>[6x]VFAEVPQAQPVLVFKLTADFREDPDPRKVNLGVGAYRTDDCHPWVLPVVKKVEQKIANDNSLNHEYLPILGLAEFRSCASRLALGDDSPALKEKRVGGVQSLGGAGALRIGADFLARWYNGTNNKNTPVYVSSPTWENHNAVFSAAGFKDIRSYRYWDAEKRGLDLQGFLNDLENAPEFSIVVLHACAHNPTGIDPTPEQWKQIASVMKHRFLFPFFDSAYQGFASGNLERDAW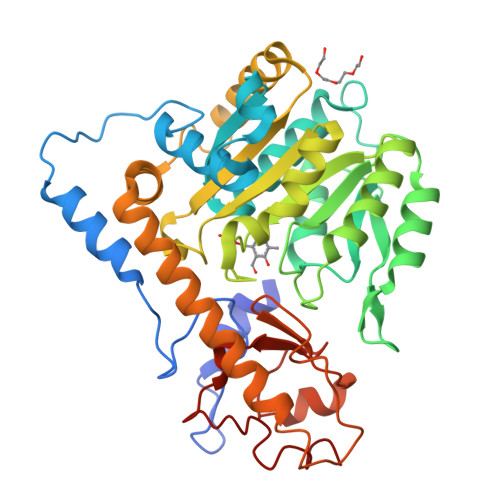AIRYFVSEGFEFFCAQSFSKNFGLYNERVGNLTVVGKEPESILQVLSQMEKIVRITWSNPPAQGARIVASTLSNPELFEEWTGNVKTMADRILTMRSELRARLEALKTPGTWNHITDQIGMFSFTGLNPKQVEYLVNEKHIYLLPSGRINVSGLTTKNLDYVATSIHEAVTKIQ> TVPDRDNDGIPDSLEVEGYTVDVKNKRTFLSPWISNIHEKKGLTKYKSSPEKWSTASDPYSDFEKVTGRIDKNVSPEARHPLVAAYPIVHVDMENIILSKNEDQSTQNTDSQTRTISKNTSTSRTHTSEVHGNAEVHASFFDIGGSVSAGFSNSNSSTVAIDHSLSLAGERTWAETMGLNTADTARLNANIRYVNTGTAPIYNVLPTTSLVLGKNQTLATIKAKENQLSQILAPNNYYPSKNLAPIALNAQDDFSSTPITMNY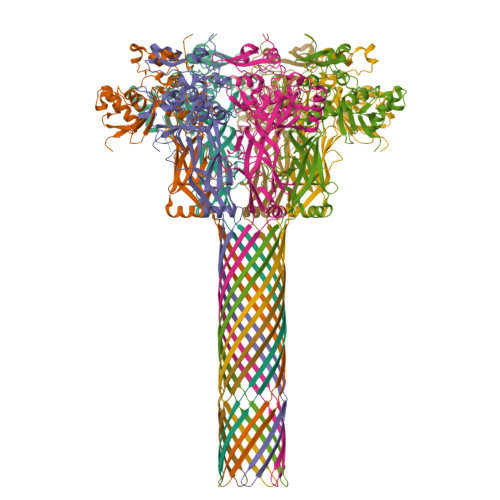NQFLELEKTKQLRLDTDQVYGNIATYNFENGRVRVDTGSNWSEVLPQIQETTARIIFNGKDLNLVERRIAAVNPSDPLETTKPDMTLKEALKIAFGFNEPNGNLQYQGKDITEFDFNFDQQTSQNIKNQLAELNATNIYTVLDKIKLNAKMNILIRDKRFHYDRNNIAVGADESVVKEAHREVINSSTEGLLLNIDKDIRKILSGYIVEIEDTEGLKEVINDRYDMLNISSLRQDGKTFIDFKKYNDKLPLYISNPNYKVNVYAVTKENTIINPSENGDTSTNGIKKILIFSKKGYEIG> MEYIIKNGFVYCPLNGVDGEKMDICVKDGKIVESVSDSAKVIDASGKIVMPGGVDPHSHIAGAKVNVGRMYRPEDSKRDAEKFKGGRAGSGFSVPSTFMTGYRYAQMGYTTAMEA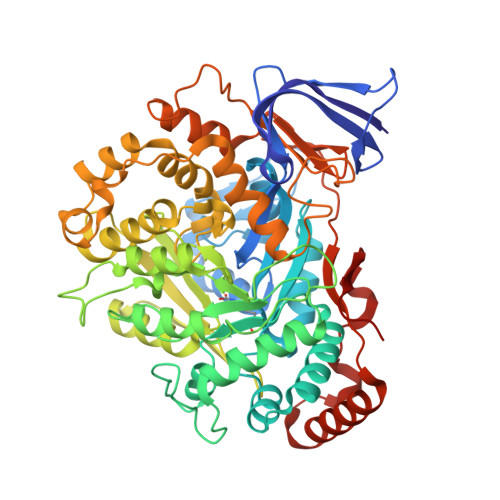AMPPLLARHTHEEFHDTPIIDHAAYPLFGNNWFVMEYLKEGDVDACAAYASWLLRATKGYTIKIVNPAGTEAWGWGGNVHGIYDPAPYFDITPAEIIKGLAEVNEKLQLPHSIHLHCNDLGHPGNYETTLASFDVPKNIKPNPATGSRDTVLYATHVQFHSYGGTTWRDFVSEAPKIADYVNKNDHIVIDVGQITLDETTTMTADGPMEYDLHSLNGLKWANCDVELETGSGVVPFIYSARAPVPAVQWAIGMELFLLIDNPEKVCLTTDSPNAGPFTRYPRVIAWLMSNKYRMNLIEGELHKWAQRKSTVATIDREYTFSEIAQITRATSAKVLGLSDTKGHLGVGADADIAVYDINPETVDPSAEYMAIEEAFSRAACVLKDGEIVVKDGEVVASPHGRTYWVDTQVDESIYSEVLANVESKFKQYYSVNFANYPVQDDYLPKSAPVKGVML> AKLGSVYTEGGFVEGVNKKLSLFGDSIDIFKGIPFAAAPKALEKPERHPGWQGTLKAKSFKKRCLQATLTQDSTYGNEDCLYLNIWVPQGRKEVSHDLPVMIWIYGGAFLMGASQGANFLSNYLYDGEEIATRGNVIVVTFNYRVGPLGFLSTGDSNLPGNYGLWDQHMAIAWVKRNIEAFGGD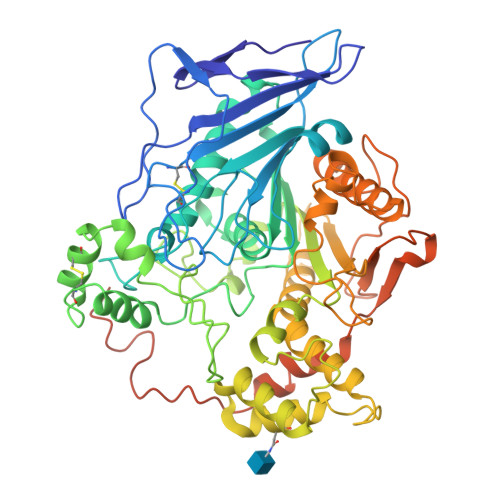PDNITLFGESAGGASVSLQTLSPYNKGLIKRAISQSGVGLCPWAIQQDPLFWAKRIAEKVGCPVDDTSKMAGCLKITDPRALTLAYKLPLGSTEYPKLHYLSFVPVIDGDFIPDDPVNLYANAADVDYIAGTNDMDGHLFVGMDVPAINSNKQDVTEEDFYKLVSGLTVTKGLRGANATYEVYTEPWAQDSSQETRKKTMVDLETDILFLIPTKIAVAQHKSHAKSANTYTYLFSQPSRMPIYPKWMGADHADDLQYVFGKPFATPLGYRAQDRTVSKAMIAYWTNFARTGDPNTGHSTVPANWDPYTLEDDNYLEINKQMDSNSMKLHLRTNYLQFWTQTYQALPTVTSAGASLLPPEDNSQASPVPPADNSGAPTEPSAGDSEVAQMPVVIGF> DIDLNKLAQRRGKHWFGTAADIPGTAETTDAAYLKVLKQNFGEITPANAMKFMYTETEQNVFNFTEGEQFLEVAERFGSKVRCHNLVWASQVSDFVTSKTWTAKELTAVMKNHIFKTVQHFGRRCYSWDVVNEA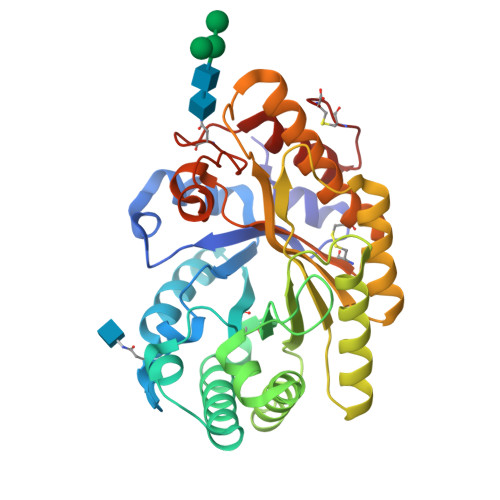LNGDGTFSSSVWYDTIGEEYFYLAFKYAQEALAQIGANDVKLYYNDYGIENPGTKSTAVLQLVSNLRKRGIRIDGVGLESHFIVGETPSLADQLATKQAYIKANLDVAVTELDVRFSTVPYYTAAAQKQQAEDYYVSVASCMNAGPRCIGVVVWDFDDAYSWVPSAFAGQGGACLFNNTLEAKPAYYAVADALEGKPCSVC> KQKPRYEIRWRVIESISPDGHEYIYVDPMQLPYDSRWEFPRDGLVLGRVLGSGAFGKVVEGTAYGLSRSQPVMKVAVKMLKPTARSSEKQALMSELKIMTHLGPHLNIVNLLGACTKSGPIYIITEYCFYGDLVNYLHKNRDSFLSHKKKSMLDSEVKNLLSDDNSEGLTLLDLLSFTYQVARG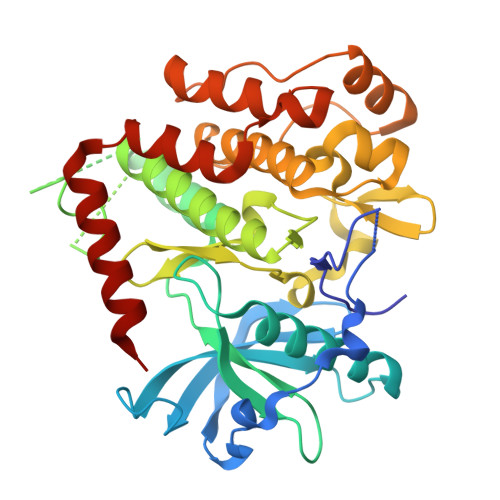MEFLASKNCVHRDLAARNVLLAQGKIVKICDFGLARDIMHDSNYVSKGSTFLPVKWMAPESIFDNLYTTLSDVWSYGILLWEIFSLGGTPYPGMMVDSTFYNKIKSGYRMAKPDHATSEVYEIMVKCWNSEPEKRPSFYHLSEIVENLLPGQYKKSYEKIHLDFLKSD5-[(2R)-1-methylpyrrolidin-2-yl]pyridin-2-ol | C10 H14 N2 O | 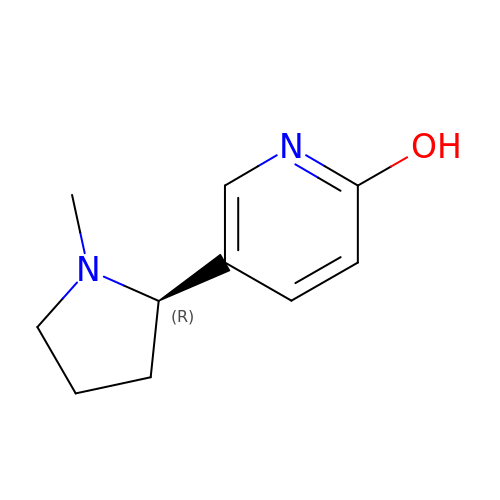ATRCOGLZUCICIV-SECBINFHSA-N> MASMTGGQQMGRDEAGITGTWYNQLGSTFIVTAGADGALTGTYESAVGNAESRYVLTGRYDSAPATDGSGTALGWTVAWKNNYRNAHSATTWSGQYVGGAEARINTQWLLTRGTTEAPAWAMTYVGHDTFTKV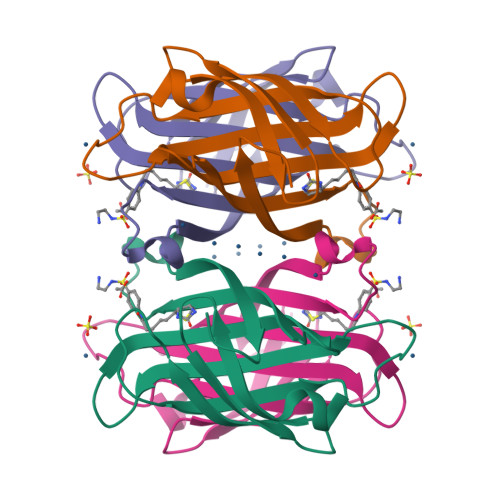KPSAASIDAAKKAGVNNGNPLDAVQQ>[2x]GSHMENMWAAEKKFSTEEEYVSPRFLVADGFLIDLAEEKPIN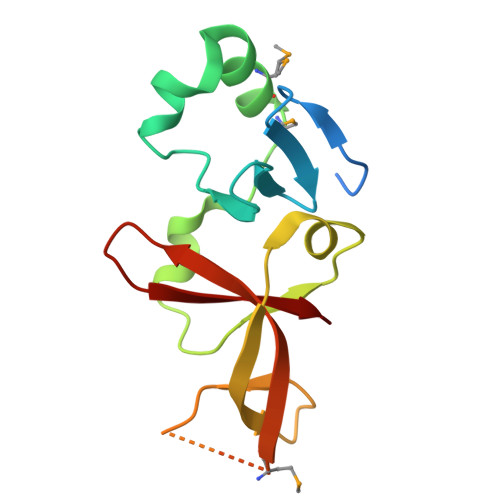PKDPRLLTLLKDHQRAMIDQMNLVKWNDFKKYQDPIPLKAKTLFKFCKQIKKKFLRGADFKLHTLPTEANLKYEPERMTVLASCVPILLDDQTVQYLYDD> ASNLKIVRMDRTA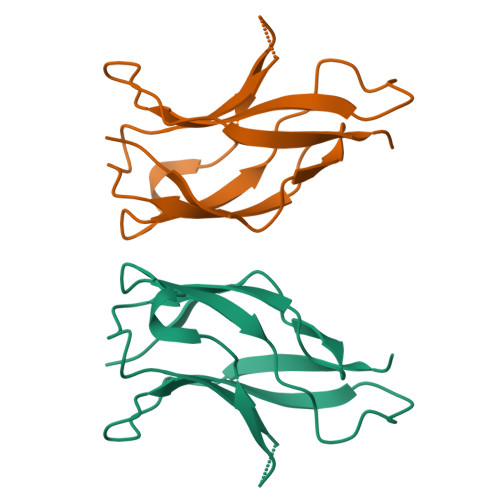GCVTGGEEIILLCDKVQKDDIQIRFYEEEENGGVWEGFGDFSPTDVHRQFAICFKTPKYKDVNITKPASVFVQLRRKSDLETSEPKPFLYYPE>[8x]KDWTQYVNPLMGSQSTFELSTGNTYPAIARPWGMNFWTPQTGKMGDGWQYTYTANKIRGFKQTHQPSPWINDYGQFSIMPIVGQPVFDEEKRASWFAHKGEVATPYYYKVYLAEHDIVTEMTPTERAVLFRFTFPENDHSYVVVDAFDKGSYIKIIPEENKIIGYTTRNSGGVPENFKNYFIIEFDKPFTYKATVENGNLQENVAEQTTDHAGAIIGFKTRKGEQVNARIASSFISFEQAAANMNELGKDNIEQLAQKGKDAWNQVLGKIEVEGGNLDQYRTFYSCLYRSLLFPRKFYELDANGQPIHYSPYNGQVLPGYMFTDTGFWDTFRCLFPLLNLMYPSVNKEMQEGLINTYLESGFFPEWASPGHRGCMVGNNSASILVDAYMKGVKVDDIKTLYEGLIHGTENVHPEVSSTG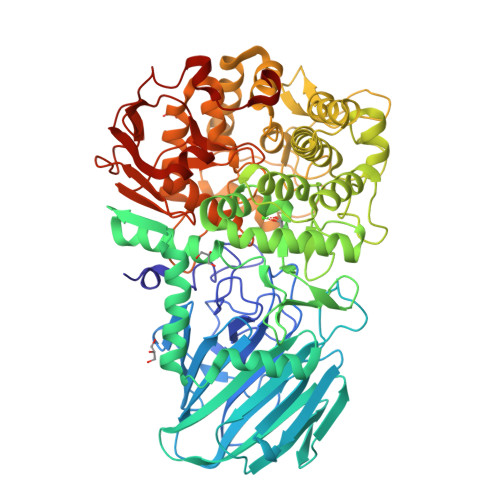RLGYEYYNKLGYVPYDVKINENAARTLEYAYDDWCIYRLAKELKRPKKEISLFAKRAMNYKNLFDKESKLMRGRNEDGTFQSPFSPLKWGDAFTEGNSWHYTWSVFHDPQGLIDLMGGKEMFVTMMDSVFAVPPIFDDSYYGQVIHEIREMTVMNMGNYAHGNQPIQHMIYLYDYAGQPWKAQYWLRQVMDRMYTPGPDGYCGDEDNGQTSAWYVFSALGFYPVCPGTDEYVMGTPLFKKATLHFENGNSLVIDAPNNSTENFYIDSMSFNGADHTKNYLRHEDLFKGGTIKVDMSNRPNLNRGTKEEDMPYSFSKELE2-hydroxy-6-methoxynaphthalene-1-carbaldehyde | C12 H10 O3 | 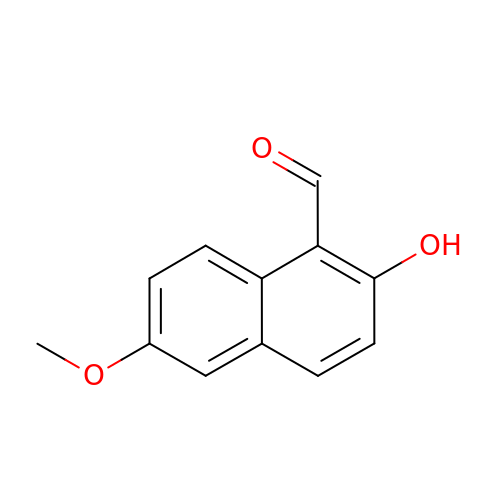OTNKCGQLSHSABI-UHFFFAOYSA-N> ASMW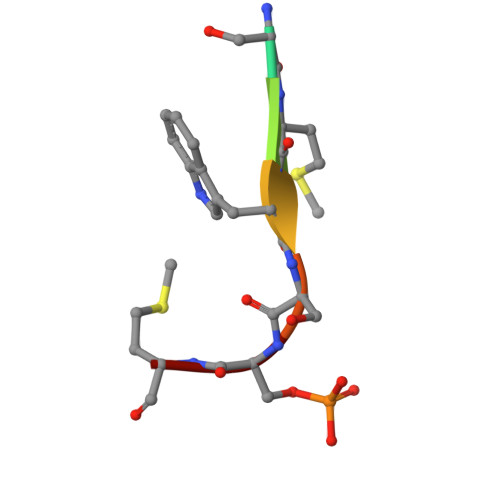SSM> MADRLTQLQDAVNSLADQFCNAIGVLQQCGPPASFNNIQTAINKDQPANPTEEYAQLFAALIARTAKDIDVLIDSLPSEESTAALQAASLYKLEEENHEAATCLEDVVYRGDMLLEKIQSALADIAQSQLKTRSGTHS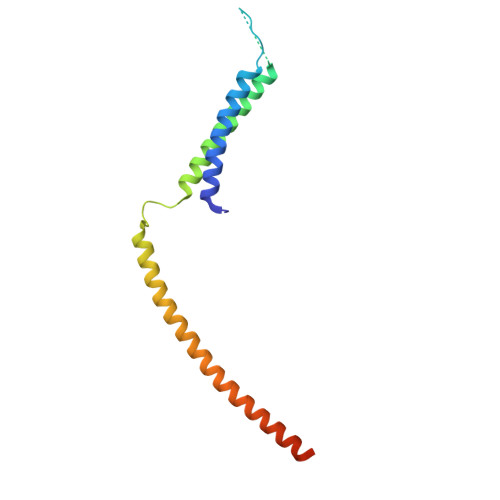QSLPDS> XGELEALAKKLKALAWKLKALSKEPSAQELEALAQELEALAKKLKALAQGX

Here, we describe the design, characterization, and application of de novo helical hairpins that heterodimerize to form 4-helix bundles in cells. Starting from a rationally designed homodimer, we construct a library of helical hairpins and identify complementary pairs using bimolecular fluorescence complementation in E. coli. We characterize some of the pairs using biophysics and X-ray crystallography to confirm heterodimeric 4-helix bundles. Finally, we demonstrate the function of an exemplar pair in regulating transcription in both E. coli and mammalian cells.

As a starting scaffold, we aimed to design a helical hairpin that homodimerized to form a 4HB. This was achieved by adapting the sequence of a previously rationally designed antiparallel homotetramer, apCC-Tet,36 and linking two helices to make a hairpin using a loop taken from a natural structure in the RSCB Protein Data Bank (PDB). The resulting peptide was called CC-HP1.0. CC-HP1.0 was soluble in aqueous buffer, and circular dichroism (CD) spectroscopy showed that it formed a stable helical assembly without an accessible thermal unfolding transition. By analytical ultracentrifugation (AUC), CC-HP1.0 formed a monodisperse dimer. However, surprisingly, the hairpins were in an anti-arrangement rather than syn. Nonetheless, the backbone of the computationally designed syn model and the experimental structure of the CC-HP1.0 dimer are similar: they both have wide and narrow helical interfaces;36 moreover, the positions of the hydrophobic-core residues overlay very well. Thus, it is possible that, due to the expected similarities of their hydrophobic cores, the syn and anti forms lie close on the free-energy landscape of these assemblies, and that under the conditions used we have crystallized out the latter. To explore this through modeling, we generated AlphaFold259−61 models using the CC-HP1.0 sequence. These predicted dimers of hairpins with the syn arrangement, i.e., as designed but in contrast to the anti-arrangement observed in the crystal structure.> MSQRIIQPSASDQQFPGKSDGYEYTVGPKQAITSEASTTYIPSRIYSESLLFKRQEASLSAMAFLFQEMISQLHRTCKTAGDFETKLSDYGHNIGIRLLELLNFRASVSPSSLPRASAFLSQNESSSKLSNASNSPGMLANSSTATSASANERLQEKQTESLSNYITKMRRRDLKILDILQFIHGTLWSYLFNHV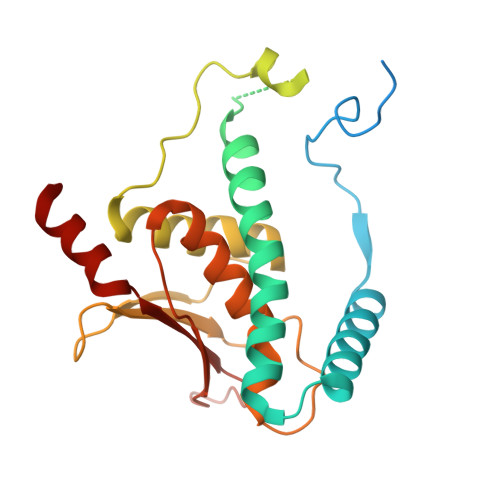SDDLVKSSERDNEYMIVDNFPTLTQFIPGENVSCEYFVCGIIKGFLFNAGFPCGVTAHRMPQGGHSQRTVYLIQFDRQVLDREGLRFG>[6x]ATPHINAEMGDFA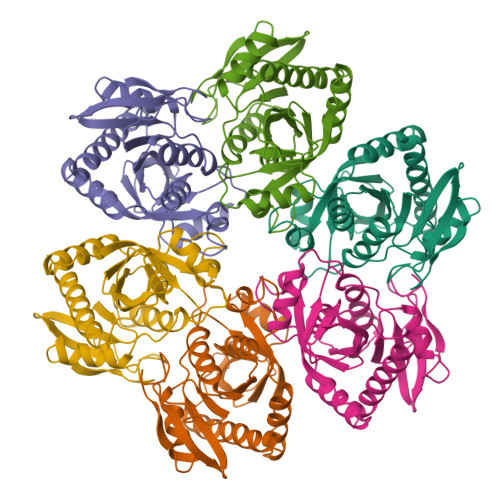DVVLMPGDPLRAKYIAETFLEDAREVNNVRGMLGFTGTYKGRKISVMGHGMGIPSCSIYTKELITDFGVKKIIRVGSCGAVLPHVKLRDVVIGMGACTDSKVNRIRFKDHDFAAIADFDMVRNAVDAAKALGIDARVGNLFSADLFYSPDGEMFDVMEKYGILGVEMEAAGIYGVAAEFGAKALTICTVSDHIRTHEQTTAAERQTTFNDMIKIALESVLLGDKE>[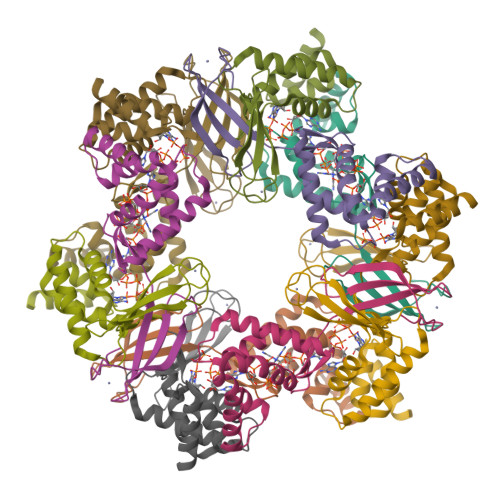12x]MHCPFCRHPDSRVVDSRTTDDGTSIRRRRQCPDCSRRFTTVETCSLMVVKRSGVTEPFSRTKVINGVRKACQGRPVTEDALAQLGQRVEEAVRATGSAELTTHDVGLAILGPLQELDLVAYLRFASVYRAFDSLEDFEAAIAELRETTGHPGEEDDTGAGSQENDRGPTGAGQVPEPAGAADKLAAALEHHHHHH>AASPPTEEAVVATEPLTREDLIAYLASGCKSKEKWRIGTEHEKFGFEVNTLRPMKYDQIAELLNSIAERFEWEKVMEGDKIIGLKQGKQSISLEPGGQFELSGAPLETLHQTCAEVNSHLYQVKAVAEEMGIGFLGMGFQPKWRREDIPTMPKGRYDIMRNYMPKVGSLGLDMMLRTCTVQVNLDFSSEADMIRKFRAGLALQPIATALFANSPFTEGKPNGFLSMRSHIWTDTDKDRTGMLPFVFDDSFGFEQYVDYALDVPMYFAYRNGKYVDCTGMTFRQFLAGKLPCLPGELPTYNDWENHLTTIFPEVRLKRYMEMRGADGGPWRRLCALPAFWVGLLYDEDVLQSVLDLTADWTPAEREMLRNKVPVTGLKTPFRDGLLKHVAEDVLKLAKDGLERRGYKEVGFL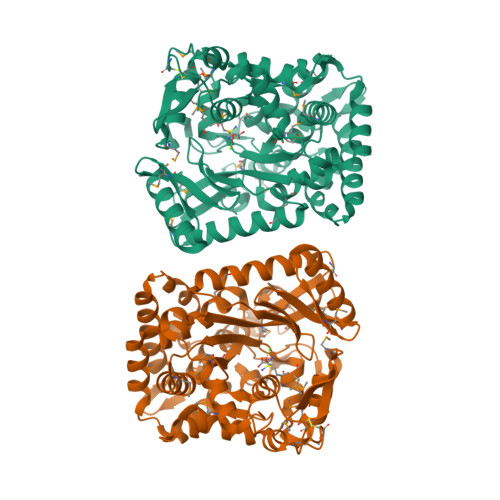NAVTEVVRTGVTPAENLLEMYNGEWGQSVDPVFQELLY[8x]>[4x]HHHHHHMQKQRTTSQWRELDAAHHLHPFTDTASLNQAGARVMTRGEGVYLWDSEGNKIIDGMAGLWCVNVGYGRKDFAEAARRQMEELPFYNTFFKTTHPAVVELSSLLAEVTPAGFDRVFYTNSGSESVDTMIRMVRRYWDVQGKPEKKTLIGRWNGYHGSTIGGASLGGMKYMHEQGDLPIPGMAHIEQPWWYKHGKDMTPDEFGVVAAR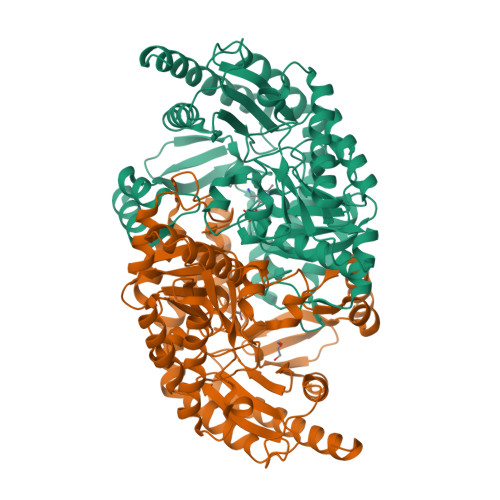WLEEKILEIGADKVAAFVGEPIQGAGGVIVPPATYWPEIERICRKYDVLLVADEVICGFGRTGEWFGHQHFGFQPDLFTAAKGLSSGYLPIGAVFVGKRVAEGLIAGGDFNHGFTYSGHPVCAAVAHANVAALRDEGIVQRVKDDIGPYMQKRWRETFSRFEHVDDVRGVGMVQAFTLVKNKAKRELFPDFGEIGTLCRDIFFRNNLIMRACGDHIVSAPPLVMTRAEVDEMLAVAERCLEEFEQTLKARGLA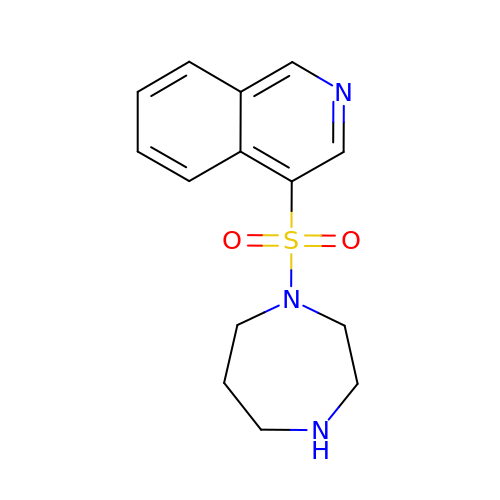4-(1,4-diazepan-1-ylsulfonyl)isoquinoline | C14 H17 N3 O2 S | YLQVZQMUQBENIS-UHFFFAOYSA-N> MAEKEEAIFRSAEMALVQFYIPQEISRDSAYTLGQLGLVQFRDLNSKVRAFQRTFVNEIRRLDNVERQYRYFYSLLKKHDIKLYEGDTDKYLDGSGELYVPPSGSVIDDYVRNASYLEERLIQMEDATDQIEVQKNDLEQYRFILQSGDEFFLKGDNTDSTSYMDEDMIDANGENIAAAIGASVNYVTGVIARDKVATLEQ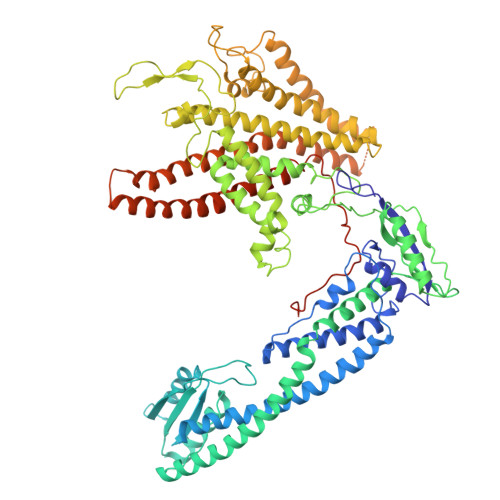ILWRVLRGNLFFKTVEIEQPVYDVKTREYKHKNAFIVFSHGDLIIKRIRKIAESLDANLYDVDSSNEGRSQQLAKVNKNLSDLYTVLKTTSTTLESELYAIAKELDSWFQDVTREKAIFEILNKSNYDTNRKILIAEGWIPRDELATLQARLGEMIARLGIDVPSIIQVLDTNHTPPTFHRTNKFTAGFQSICDCYGIAQYREINAGLPTIVTFPFMFAIMFGDMGHGFLMTLAALSLVLNEKKINKMKRGEIFDMAFTGRYIILLMGVFSMYTGFLYNDIFSKTMTIFKSGWKWPDHWKKGESITATSVGTYPIGLDWAWHGTENALLFSNSYKMKLSILMGFIHMTYSYFFSLANHLYFNSMIDIIGNFIPGLLFMQGIFGYLSVCIVYKWAVDWVKDGKPAPGLLNMLINMFLSPGTIDDELYPHQAKVQVFLLLMALVCIPWLLLVKPLHFKFTHKKKSHEPLPSTEADASSEDLEAQQLISAMDADDAEEEEVGSGSHGEDFGDIMIHQVIHTIEFCLNCVSHTASYLRLWALSLAHAQLSSVLWTMTIQIAFGFRGFVGVFMTVALFAMWFALTCAVLVLMEGTSAMLHSLRLHWVESMSKFFVGEGLPYEPFAFEYKDMEVAVASASSSASSDYKDHDGDYKDHDIDYKDDDDK>AARSSIVLTDGTTPVTLTPVGGGVGQTLYRATAEALSAANPSLSFGYRFTDGGTNRQSLSYKQPITAVDSTTSETLVRGQCVVDINIVIPRVATATDR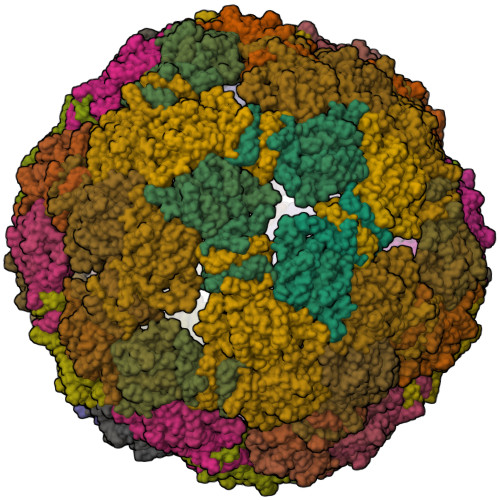AEAIKRAFDVLNALNAELITGEGQW[180x]>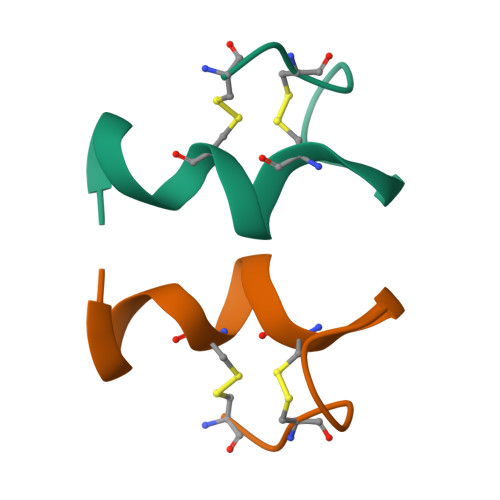 CSCSSLMDKECVYFCHLDIIW>MSMKQRVIIVGGGPVGLLTALGLAKAGTNVVVLEAESQPSDSPRALVYHFPVLPHLKRLGVLDDCVAAGLMRQNFAWRVHSTSEMIFWDLSCLEGDVELPYALHLGQDKLSRILIEHLKALPNVEVRYSSPVVDCEVGPRSVRVVLGGESPGVIVEGDWLIGADGANSFVRREVLNQNFFGITWPQRYVATNTRFDFDKLGFGKTTMQVDDVYGSVICNIDADSLWRVTFMEDPNLPMEGIRGRIDQVFKELLPTNDPYEVVAFSPYRMHQ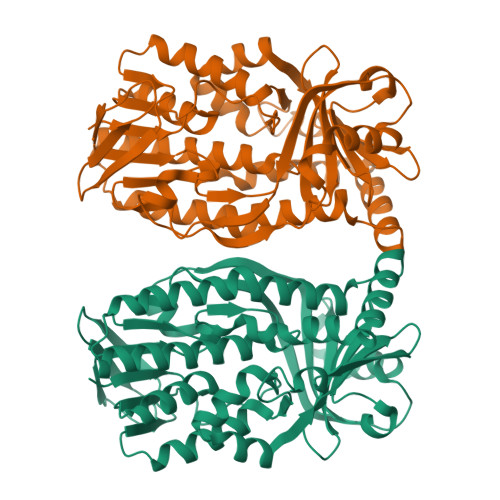RVTDRMRNGRVILIGDAAHVTNPTGGLGLTGGMFDAFALTSVLNQVIHDGRSEDILDVFEADRRRKFIELVSPRASDNLRNLYHQKPGEGKNDWVNNTRSISKDIDRMRDALRFPETMETFL[2x]>[8x]MRGIILAGGSGTRLYPITMGISKQLLPVYDKPMIYYPLTTLMMAGIRDIQLITTPHDAPGFHRLLGDGAHLGVNISYATQDQPDGL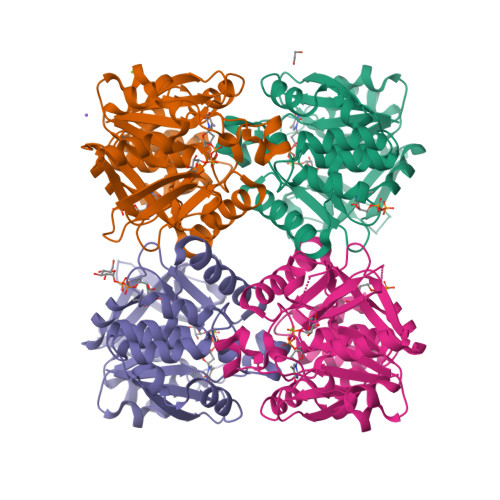AQAFVIGANHIGADSVALVLGDNIFYGPGLGTSLKRFQSISGGAIFAYWVANPSAYGVVEFGAEGMALSLEEKPVTPKSNYAVPGLYFYDNDVIEIARGLKKSARGEYEITEVNQVYLNQGRLAVEVLARGTAWLDTGTFDSLLDAADFVRTLERRQGLKVSIPEEVAWRMGWIDDEQLVQRARALVKSGYGNYLLELLERNLEHHHHHH> MTKTGTDYSAWSELTSSVNTSVSGIVDLASLTFTT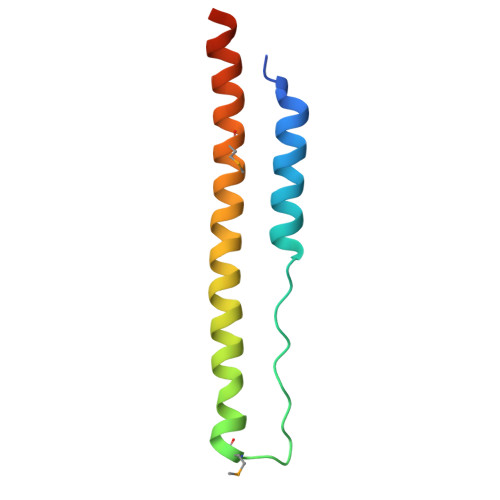TTMTPFTSFNEDISSFNTAVAKLQSFTSTDVTHMNQAAENKVTDDSNQAQAQG> ASMKQPVVVIGSGLAGLTTSNRLISKYRIPVVLLDKAASIGGNSIKASSGINGAHTDTQQNLKVMDTPELFLKDTLHSAKGRGVPSLMDKLTKESKSAIRWLQTEFDLKLDLLAQLGGHSVPRTHRSSGKLPPGFEIVQALSKKLKDISSKDSNLVQIMLNSEVVDIELDNQGHVTGVVYMDENGNRKIMKSHHVVFCSGGFGYSKEMLKEYSPNLIHLPTTNGKQTTGDGQKILSKLGAELIDMDQVQVHPTGFIDPNDRENNWKFLAAEALRGLGGILLHPTTGRRFTNELSTRDTVTMEIQSKCPKNDNRALLVMSDKVYENYTNNINFYMSKNLIKKVSINDLIRQYDLQTTASELVTELKSYSDVNTKDTFDRPLIINAFDKDISTESTVYVGEVTPVVHFTMGGVKINEKSQVIKKNSESVLSNGIFAAGEVSGGVHGANRLGGSSLLECVVFGKTAADNIAKLY

Fumarate reductase is a flavoprotein enzyme containing the cofactor flavin adenine dinucleotide (FAD) that is responsible for reducing fumarate to succinate. Two soluble fumarate reductases, Frd1 and Osm1, which are essential for anaerobic growth, have been identified in Saccharomyces cerevisiae. Interestingly, a sequence comparison within the Fcc3 family has suggested that both Osm1 and Frd1 contain only a flavin domain and a clamp domain, and thus lack the cytochrome domain, which is critical for electron transfer. In the current study, we provide two structures for Osm1: one in a complex with its cofactor (FAD) and substrate (fumarate), and another in a complex with its cofactor FAD, substrate, and a second unexpected FAD molecule located in a newly defined second FAD-binding pocket.

Following an intensive effort to overcome these purification and crystallization issues, we finally solved the 1.8 Å crystal structure of Osm1. The asymmetric unit contained one molecule, with the final model encompassing residues 32–501. The Osm1 structure contained the FAD cofactor and the fumarate substrate in the active site. The high-resolution structure of Osm1, in the presence of its cofactor and substrate, revealed that it comprises 17 helices, α1–α17, and 19 β-sheets, β1–β19, forming two distinct domains, a flavin domain (residues 32–268 and 386–501) and a clamp domain (residues 269–385). The FAD- and substrate-bound active site is located in the center of the protein at the interface of the two domains, each lining part of the active site. Fifteen amino acid residues, including A45, K66, N73, S74, S79, G80, V194, D260, E467, S482, and L483, from the flavin domain form hydrogen bonds of 3.5 Å or less with the FAD cofactor. Fumarate is located immediately next to the isoalloxazine ring of the FAD cofactor, having a direct interaction with the protein. S78, S79, H281, R326, H435, R477, and G480 from Osm1 are involved in the binding of fumarate in the active site through the formation of hydrogen bonds. Based on our analysis using SEC-MALS, we conclude that FAD- and substrate-bound Osm1 exists as a monomer in solution. Compared to the structures of other prokaryotic soluble fumarate reductases from the Fcc3 family, the most notable feature of the Osm1 structure was that it did not contain a heme domain, which is known to be critical for electron transfer.> MGDLSCPEGLEELLSAPPPDLGAQRRHGWNPKDCSENIEVKEGGLYFERRPVAQSTDGARGKRGYSRGLHAWEISWPLEQ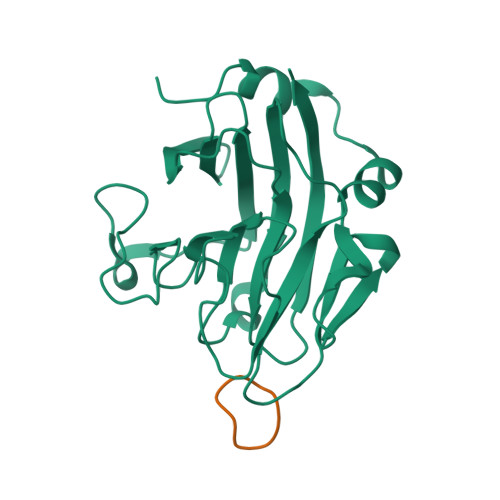RGTHAVVGVATALAPLQTDHYAALLGSNSESWGWDIGRGKLYHQSKGPGAPQYPAGTQGEQLEVPERLLVVLDMEEGTLGYAIGGTYLGPAFRGLKGRTLYPAVSAVWGQCQVRIRYLGERGSHHHHHH;> RGDINNNV> LYFQGNMK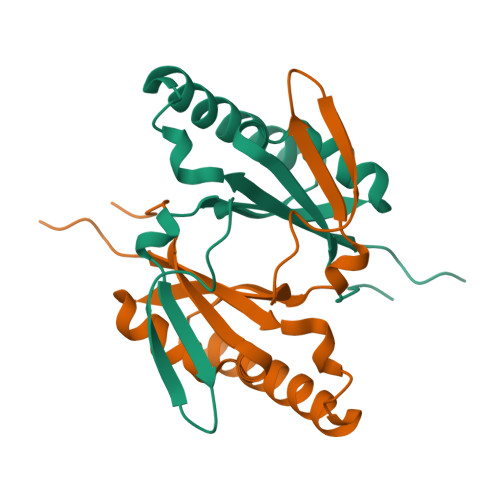YLCLIYFDEAKLAAVPAEELAAIVDECMTYSDQLGKAGHYIASHALQSVQTATTLRHQGGRLAMTDGPFAETKEQLGGFYLIEARDLNQALQIAAKIPPGRLGCVEVRPVKEWEGS> IEEVMKTVANTVESEIRAELGVIPSLNAAETGATSNTTPEEAIQTRAVINQHGTSETLVENFLGRAALVMMKDFEYKNHVTGTQKVQQNFFKWTINTRSYVQLRRKFELFTYIRFDSEITIVPTIRLYTSTGASYSGLPNLTLQAMFVPVGAPTPKSQDSYEWQSACNPSVFFKIDDPPARMTIPFMCINSAYGMFYDGFAGFEKTANGLYGINPANTMGNLCIRVVNAYQPVQYTITIRIYLKPKHIKAWVPRPPRTMPYMSIANTNYTGHSSAPNNVNAIVGNRTNITTMPNDIV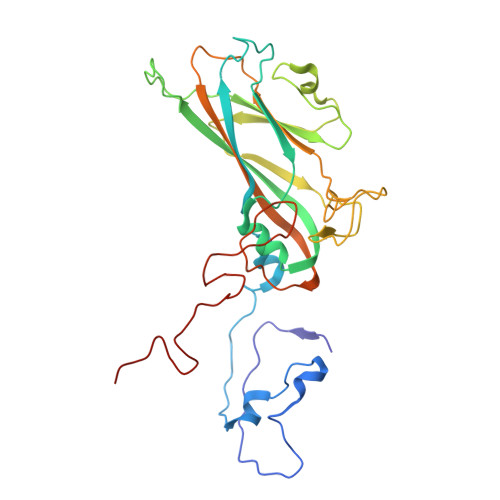T(2S)-2-[(E)-3-[2-(diethylamino)ethyl-[[4-[4-(trifluoromethyl)-2-[2,2,2-tris(fluoranyl)ethoxy]phenyl]phenyl]methyl]amino]-1-oxidanyl-3-oxidanylidene-prop-1-enyl]pyrrolidine-1-carboxylic 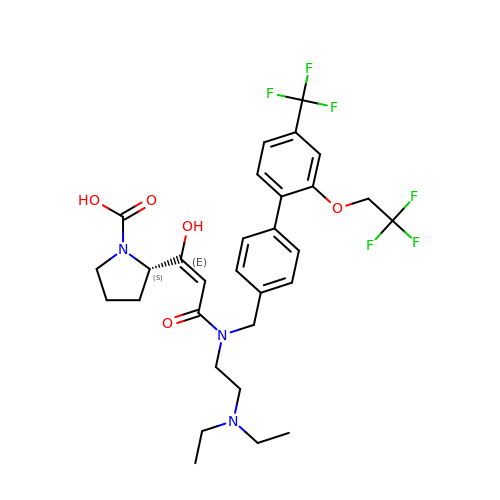acid | C30 H35 F6 N3 O5 | MYCHXHCCMGJMEM-IOCYEQIYSA-N The ESCRT-III-like protein Vipp1 couples filament polymerization with membrane remodeling. It assembles planar sheets as well as 3D rings and helical polymers, all implicated in mitigating plastid-associated membrane stress. PspA activity is triggered by agents that threaten inner membrane integrity, including phage, mislocalized secretins, and antibiotics, whereas Vipp1 is a plastid component in cyanobacteria, algae, and plants, in which it functions in thylakoid membrane biogenesis and repair. Given that two-dimensional (2D) planar sheets share a close geometric relationship with helical lattices, and as a means of understanding the interconnectedness of Vipp1 polymers including rings, spirals and planar sheets, we determined the structure of four Vipp1 helical filaments by cryo-EM.

Alternatively, Vipp1Δα61–219 assembled with related but different lattices, termed Vipp1Δα6_L2 and Vipp1Δα6_L3. Specifically, Vipp1Δα61–219 purified in low-salt conditions (10 mM NaCl), has a greater propensity to form ordered helical filaments and quasi-helical ring stacks than does Vipp1. The structure of Vipp1Δα6_L2 was very similar to that of Vipp1Δα6_L3, although different helical parameters yielded a modified helical lattice with a slight lattice rotation relative to the helical axis. Specifically, the left-handed 21-start helix in Vipp1Δα6_L2 and Vipp1Δα6_L3 that runs nearly parallel to the helix axis formed a 19-start helix in Vipp1L1. The CTD modulates Vipp1 polymer stability and dynamism and in its absence, Vipp1 has a higher avidity to form polymers with increased regularity and stability.

> MGLFDRIKRVVSSNLNDLVNKAEDPEKMLEQAILEMQEDLVQLRQGVAQAIAAQKRSEKQYNDAQNEINKWQRNAQLALQKGDENLARQALERKKTYTDTSAALKASLDTQSTQVETLKRNLIQLESKISEAKTKKEMLKARITTAKAQEQLQGMVRGMNTSSAMSAFERMEEKVLMQESRAQALGELAGADLETQFAQLEGGSDVDDELAALKAQM[(2R,3R,4R,5R)-5-(6-AMINO-9H-PURIN-9-YL)-3-HYDROXY-4-(PHOSPHONOOXY)TETRAHYDROFURAN-2-YL]METHYL [(2R,3S,4S)-3,4-DIHYDROXYTETRAHYDROFURAN-2-YL]METHYL 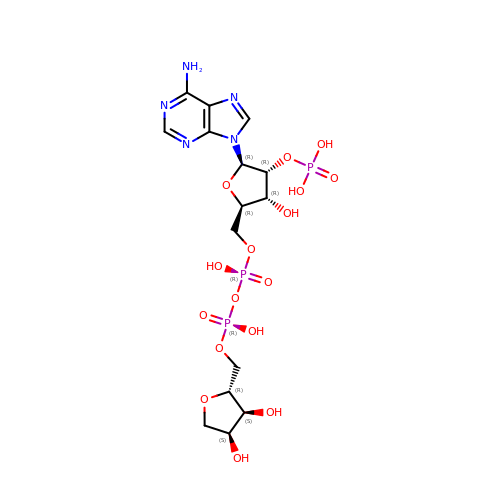DIHYDROGEN DIPHOSPHATE | C15 H24 N5 O16 P3 | XDDBFIXGEVGCEU-AOOZFPJJSA-N> DEV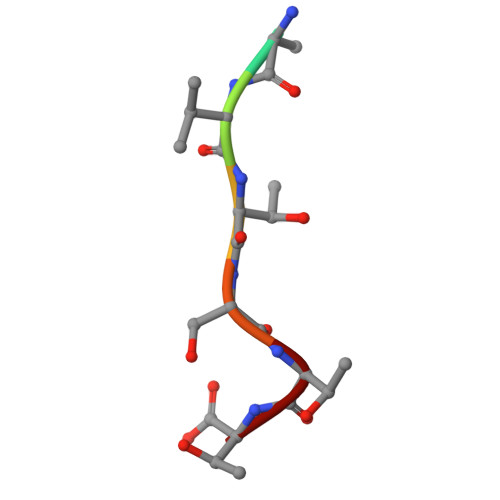TSTT> SNAMKATRLAIPDVILFEPRVFGDDRGFFFESY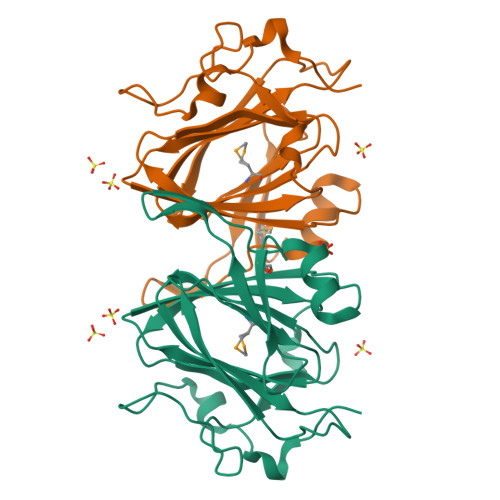NQRAFEEACGHPVSFVQDNHSRSARGVLRGLHYQIRQAQGKLVRATLGEVFDVAVDLRRGSPTFGQWVGERLSAENKRQMWIPAGFAHGFVVLSEYAEFLYKTTDFWAPEHERCIVWNDPELKIDWPLQDAPLLSEKDRQGKAFADADCFP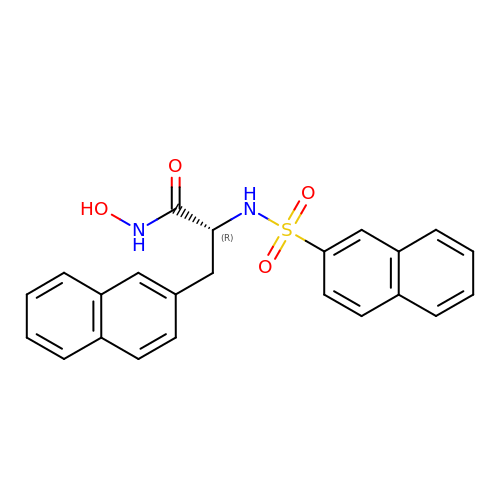(2R)-N-hydroxy-3-naphthalen-2-yl-2-[(naphthalen-2-ylsulfonyl)amino]propanamide | C23 H20 N2 O4 S | MMOUXLMPQFMDRD-JOCHJYFZSA-N>[8x]MASRGSHHHHHHGAYRLLNKTAVITGGGSGIGLATAKRFVAEGAYVFIVDVSRKELEQAAAEIGRNVTAVKADVTKLEDLDRLYAIVREQR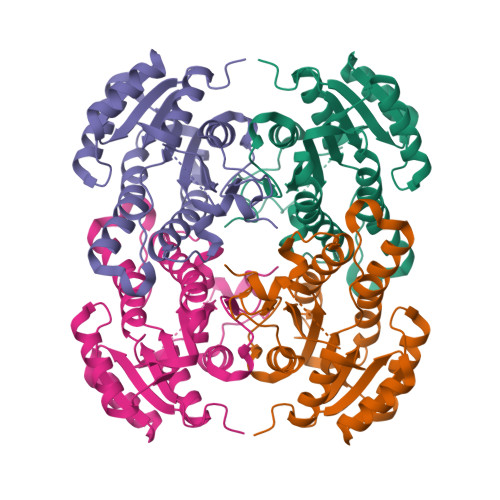GSIDVLFNNAGAIEQKTLEEITPEHYDRTFDVNVRGLIFTVQKALPLLRDGGSVILTSSVAGVLGLQAHDTYSAAKAAVRSLARTWTTELKGRSIRVNAVSPGAIDTPIIENQVSTQEEADELRAKFAAATPLGRVGRPEELAAAVLFLASDDSSYVAGIELFVDGGLTQV> AA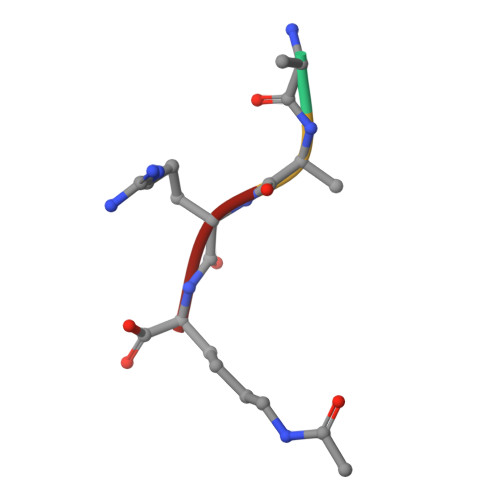RK ETHYLISOTHIOUREA | C3 H8 N2 S 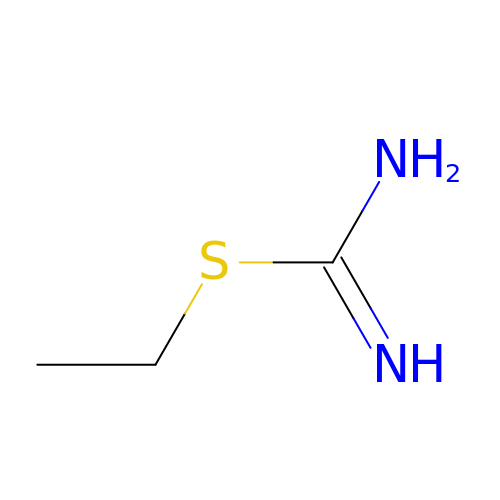| VFIZBHJTOHUOEK-UHFFFAOYSA-N> NTQAKTFVRSQLFPEEMPQFLEKKKQVGILGGTFNPVHLAHLVMAEQAGRNLGLDRVFLMPSYQPPHVDEKQTIDAKHRLNMLELAVEDNPFLQIETIELARGGKSYTYDTMKELTQNNPDTDYYFIIGGDM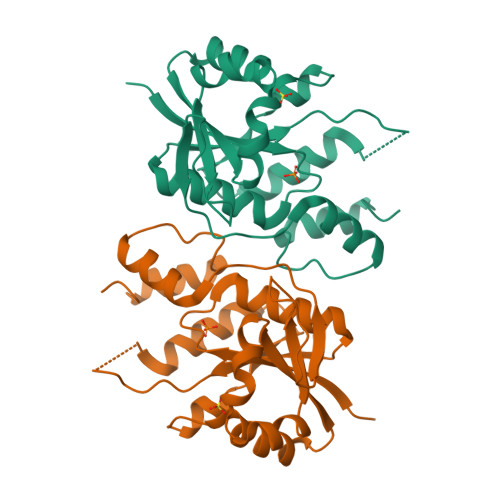VEYLPKWYKIDELTSMVNFVGIRRPGYTTDTPYPVIWVDVPEIDISSTKIRQKIKEGCSIRYLVPDKVIDYIQNEGLYEYGL> MAKNKIPNSRLMINYETNVDGVLKKKELPYRVLVVGDLSKGRSVDAKKEFADREVRRVN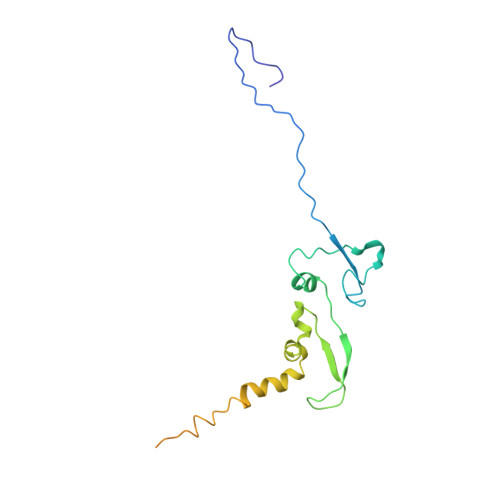NGVDRVLEEMNISFDFEAPNFVSKDPSNLKVNYRIESVKDFRPDAVAKKVPEIRALLEMKEILASFAKDIENNRNLKKTIDMIFSDSNELESLKSKIPALTNYTIKDSCDAAESQDLSNQQVDDK Hapalindole U | C21 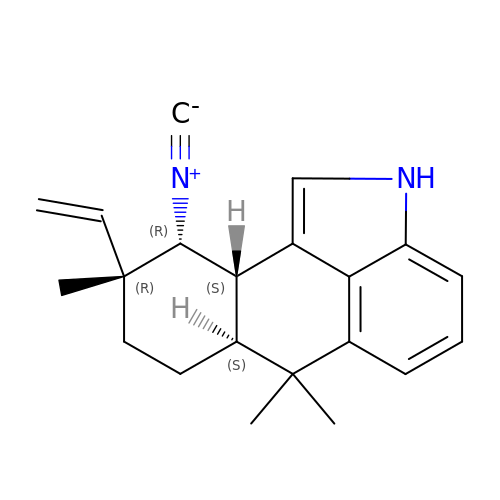H24 N2 | SLUFHMQYBPOTFZ-ZRRCRCOKSA-N>[2x]MGTVSSRRSWWPLPLLLLLLLLLGPAGARAQEDEDGDYEELVLALRSEEDGLAEAPEHGTTATFHRCAKDPWRLPGTYVVVLKEETHLSQSERTARRLQAQAARRGYLTKILHVFHGLLPGFLVKMSGDLLELALKLPHVDYIEEDSSVFAQSIPWNLERITPPRYRADEYQPPDGGSLVEVYLLDTSIQSDHREIEGRVMVTDFENVPEEDGTRFHRQASKCDSHGTHLAGVVSGRDAGVAKGASMRSLRVLNCQGKGTVSGTLIGLEFIRKSQ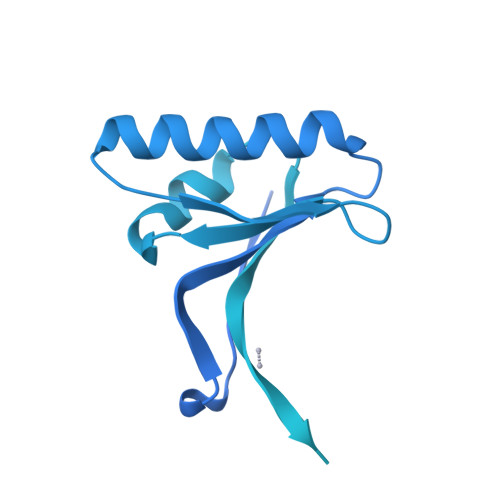LVQPVGPLVVLLPLAGGYSRVLNAACQRLARAGVVLVTAAGNFRDDACLYSPASAPEVITVGATNAQDQPVTLGTLGTNFGRCVDLFAPGEDIIGASSDCSTCFVSQSGTSQAAAHVAGIAAMMLSAEPELTLAELRQRLIHFSAKDVINEAWFPEDQRVLTPNLVAALPPSTHGAGWQLFCRTVWSAHSGPTRMATAIARCAPDEELLSCSSFSRSGKRRGERMEAQGGKLVCRAHNAFGGEGVYAIARCCLLPQANCSVHTAPPAEASMGTRVHCHQQGHVLTGCSSHWEVEDLGTHKPPVLRPRGQPNQCVGHREASIHASCCHAPGLECKVKEHGIPAPQEQVTVACEEGWTLTGCSALPGTSHVLGAYAVDNTCVVRSRDVSTTGSTSEEAVTAVAICCRSRHLAQASQELQ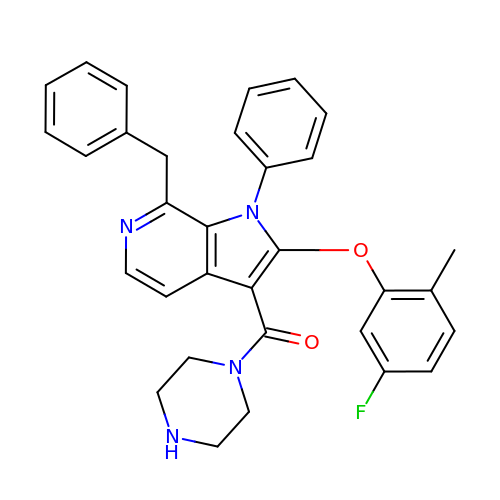[7-benzyl-2-(5-fluoro-2-methylphenoxy)-1-phenyl-1H-pyrrolo[2,3-c]pyridin-3-yl](piperazin-1-yl)methanone | C32 H29 F N4 O2 | UIBPLELQTBSRIZ-UHFFFAOYSA-N> AGCATGA;> CAATGACTCATGCTCATCGGA;>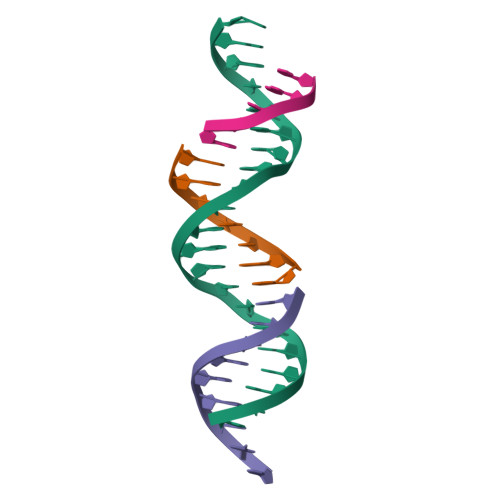 TGTCCGATG;> GTCAT>GAMDPSPNYDKWEMERTDITMKHKLGGGQYGEVYEGVWKKYSLTVAVKTLKEDTMEVEEFLKEAAVMKEIKHPNLVQLLGVCTREPPFYIITEFMTYGNLLDYLRECNRQEVNAVVLLYMATQISSAMEYLEKKNFIHRDLAARNCLVGENHLVKVADFGLSRLMTGDTYTAHAGAKFPIKWTAPESLAYNKFSIKSDVWAFGVLLWEIATYGMSPYPGIDLSQVYELLEKDYRMERPEGCPEKVYELMRACWQWNPSDRPSFAEIHQAFETMFQE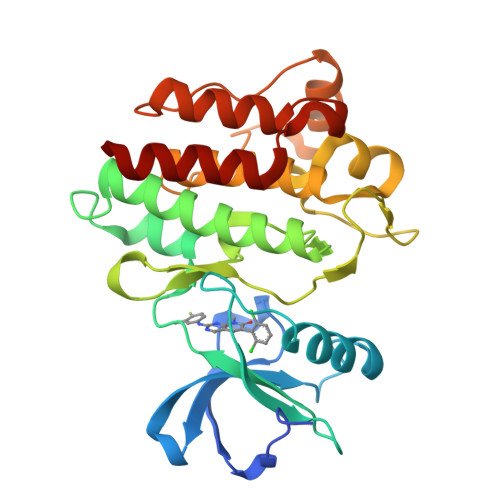S[2x]> GSHEQFRAALQLVVDPGDPRSYLDNFIKIGE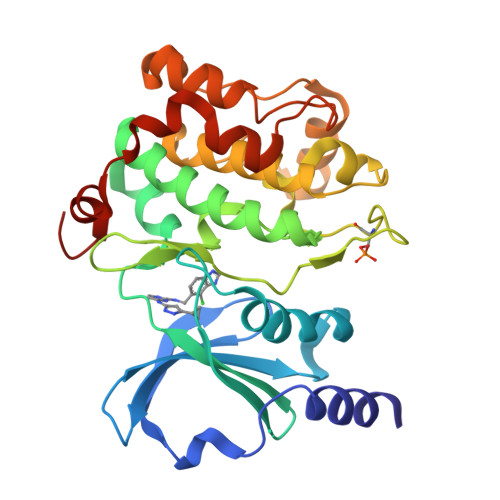GSTGIVCIATVRSSGKLVAVKKMDLRKQQRRELLFNEVVIMRDYQHENVVEMYNSYLVGDELWVVMEFLEGGALTDIVTHTRMNEEQIAAVCLAVLQALSVLHAQGVIHRDIKSDSILLTHDGRVKLSDFGFCAQVSKEVPRRKSLVGTPYWMAPELISRLPYGPEVDIWSLGIMVIEMVDGEPPYFNEPPLKAMKMIRDNLPPRLKNLHKVSPSLKGFLDRLLVRDPAQRATAAELLKHPFLAKAGPPASIVPLMRQNRTR S-ribosylhomocysteine | C9 H17 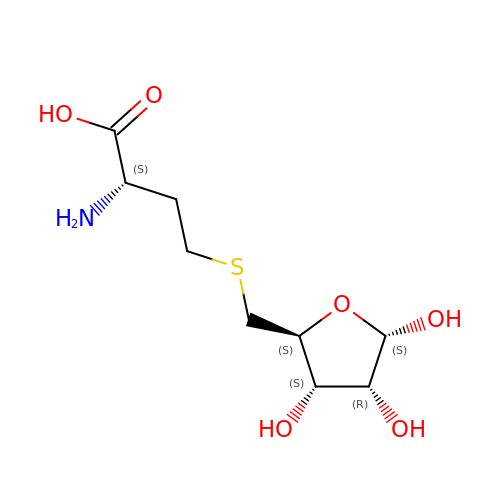N O6 S | IQFWYNFDWRYSRA-LYNCRYNASA-N> ESPLPKPVLDTNGKELNPDSSYRIIS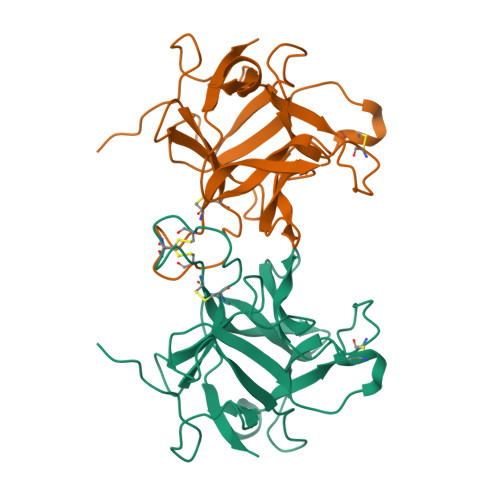IGRGALGGDVYLGKSPNSDAPCPDGVFRYNSDVGPSGTPVRFIPLSTNIFEDQLLNIQFNIPTVKLCVSYTIWKVGNLNAYFRTMLLETGGTIGQADNSYFKIVKSSKIGYNLLSCPFTSIICLRCPEDQFCAKVGVVIQNGKRRLALVNENPLDVLFQEV>MTGSNSHITILTLNINGLNSAIKRHRLASWIKSQDPSVCCIQETHLTCRDTHRLKIKGWRKIYQANGKQKKAGVAILVSDKTDFKPTKIKRDKEGHYIMVKGSIQQEELTILNIYAPNTGAPRFIKQVLSDLQRDLDSHTLIMGDFNTPLSTLDRSTRQKVNKDTQELNSALHQADLIDIY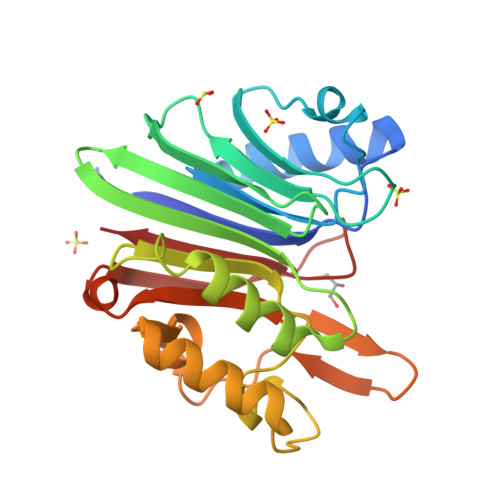RTLHPKSTEYTFFSAPHHTYSKIDHIVGSKALLSKCKRTEIITNYLSDHSAIKLELR[2x]>RLYWDDLKRKLSEKLDSTDFTSTIKLLNENSYVPREAGSQKDENLALYVENQFREFKLSKVWRDQHFVKIQVKDSAQNSVIIVDKNGRLVYLVENPGGYVAYSKAATVTGKLVHANFGTKKDFEDLYTPVNGSIVIVRAGKITFAEKVANAESLNAIGVLIYMDQTKFPIVNAELSFFGHAHLGTGDPYTPGFPSFNHTQFPPSRSSGLPNIPVQTISRAAAEKLFGNMEGDCPSDWKTDSTCRMVTSESKNVKLTVSNVLKEIKILNIFGVIKGFVEPDHYVVVGAQRDAWGPGAAKSGVGTALLLKLAQMFSDMVLKDGFQPSRSIIFASWSAGDFGSVGATEWLEGYLSSLHLKAFTYINLDKAVLGTSNFKVSASPLLYTLIEKTMQNVKHPVTGQFLYQDSNWASKVEKLTLDNAAFPFLAYSGIPAVSFCFCEDTDYPYLGTTMDTYKELIERIPELNKVARAAAEVAGQFVIKLTHDVELNLDYERYNSQLLSFVRDLNQYRADIKEMGLSLQWLYSARGDFFRATSRLTTDFGNAEKTDRFVMKKLNDRVMRVEYHFLSPYVSPKESPFRHVFWGSGSHTLPALLENLKLRKQNNGAFNETLFRNQLALATWTIQGAANALSGDVWDIDNEF[2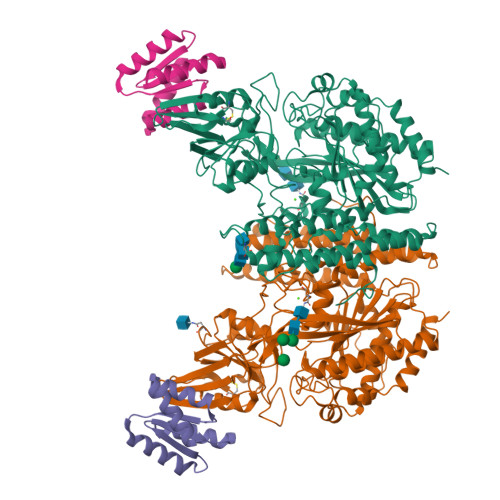x];>[2x]DEEEIQKAIEELLRKGVSEEEAAIIIVQRFNVAVVVVVQDERQAKHISEYIRRYIPEADVILFANIVVIKVETHELRKRVWEAAQKAY>APVRSLNCRIWDVNQKTFYLRNNQLVAGYLQGPNVNLEEKFSMSFVQGEESNDKIPVALGLKEKNLYLSCVLKDDKPTLQLESVDPKNYPKKKMEKRFVFNKIEINNKLEFESAQFPNWFLCTAMEADQPVS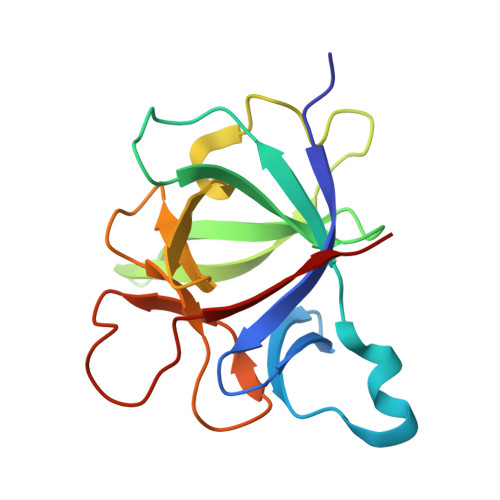LTNMPDEGVMVTKFYMQFVSS[2x]> MASSINPWILTGFADAEGSFILRIRNNNGMRVGYLTELIFSIKLHNKDKSILENIQSTWKVGKITNNGDQAVMLRVSRFEDLKVIIDHFEKYPLITQKLGDYKLFKQAYSVMENKEH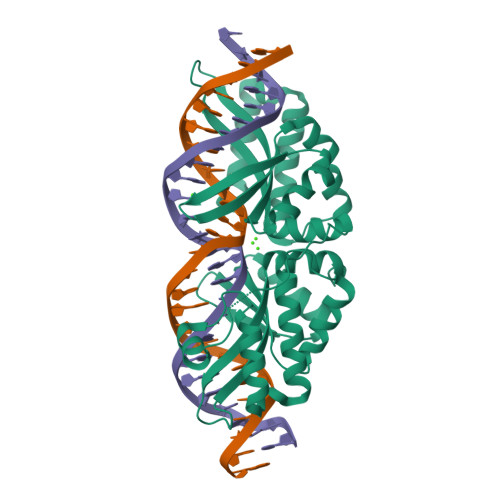LKENGIKELVRIKAKMNWGLTDELKKAFPEIISKERPLINKNIPNLKWLAGFTSGEGHFGVNLWKRKGGTHVGVQLVFGISQHIRDKNLMNSLITYLGCGYILEKNRSELSWLDFRVTKFSDINDKIIPVFQENTLIGVKLEDFEDWCKVAKLIEEKKHLTESGLDEIKKIKLNMNKGR>[4x]SQSFLLKSLEQVRKIQ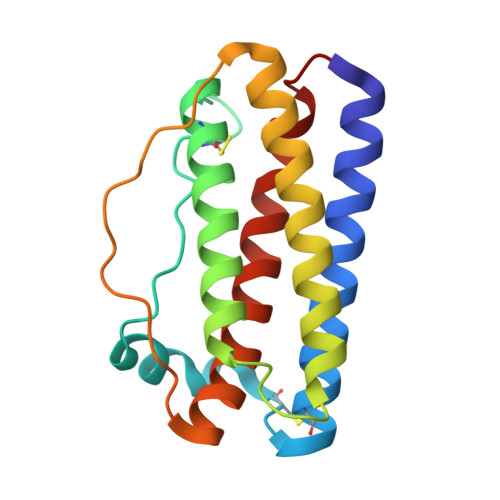GDGAALQEKLCATYKLCHPEELVLLGHSLGIPWAPLSSCPSQALQLAGCLSQLHSGLFLYQGLLQALEGISPELGPTLDTLQLDVADFATTIWQQMEELGMAPALQPTQGAMPAFASAFQRRAGGVLVASHLQSFLEVSYRVLRHLG>[2x]PNFSGNWKIIRSENFEELLKVLGVNVMLRKIAVAAASKPAVEIKQEGDTFYIKTSTTVRTTEINFKVGEEFE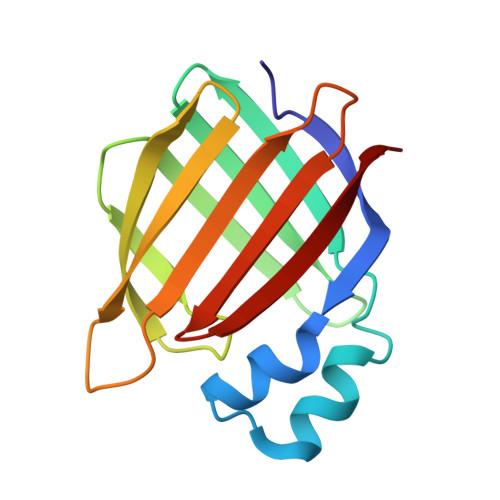EQTVDGRPCKSLVKWESENKMVCEQKLLKGEGPKTSWTLELTNDGELILTMTADDVVCTKVYVRE> LQTA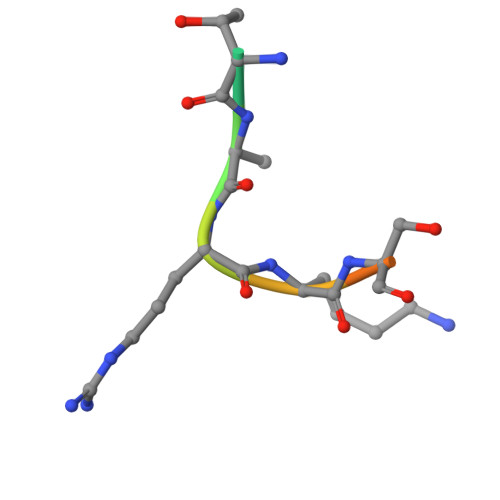RKSTGG> XSLSSKLSVQDLDLKDKRVFIRVDFNVPLDGKKITSNQRIVAALPTIKYVLEHHPRYVVLASHLGRPNGERNEKYSLAPVAKELQSLLGKDVTFLNDCVGPEVEAAVKASAPGSVILLENLRYHIEEEGSRKVDGQKVKASKEDVQKFRHELSSLADVYINDAFGTAHRAHSSMVGFDLPQRAAGFLLEKELKYFGKALENPTRPFLAILGGAKVADKIQLIDNLLDKVDSIIIGGGMAFTFKKVLENTEIGDSIFDKAVGPEIAKLMEKAKAKGVEVVLPVDFIIADAFSASANTKTVTDKEGIPAGWQGLDNGPESRKLFAATVAKATVILWNGPPGVFEFEKFAAGTKALLDEVVKSSAAGNTVIIGGGDTATVAKKYGVTD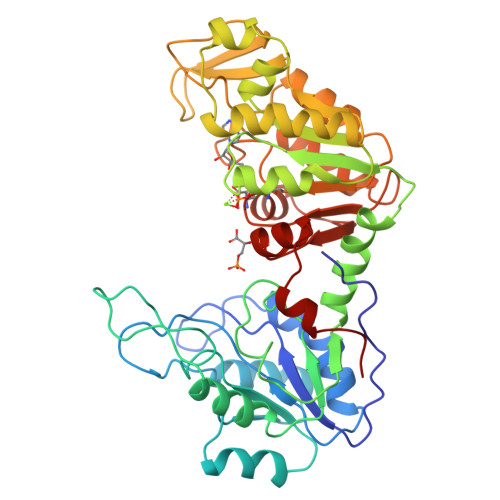KISHVSTGGGASLELLEGKELPGVAFLSEKK>[2x]LNEQVNYTPQQRQYLESFIEKYVDKTKGSKQYTDETRFAHANNRNLSSFRSYWKEMVYP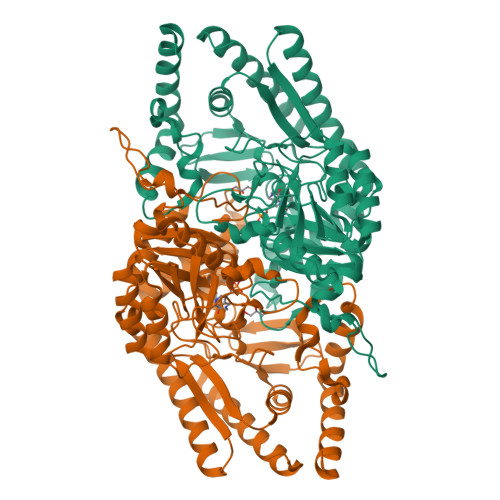IIAERSDGSRMWDIDGNEYIDITMGFGVNLFGHHPSFITQTVVDSTHSALPPLGPMSNVAGEVADRIRACTGVERVAFYNSGTEAVMVALRLARAATGRTKVVVFAGSYHGTFDGVLGVANTKGGAEPANPLAPGIPQSFMNDLIILHYNHPDSLDVIRNLGNELAAVLVEPVQSRRPDLQPESFLKELRAITQQSGTALIMDEIITGFRIGLGGAQEWFDIQADLVTYGKIIGGGQPLGIVAGKAEFMNTIDGGTWQYGDDSYPTDEAKRTFVAGTFNTHPLTMRMSLAVLRYLQAEGETLYERLNQKTTYLVDQLNSYFEQSQVPIRMVQFGSLFRFVSSVDNDLFFYHLNYKGVYVWEGRNCFLSTAHTSDDIAYIIQAVQETVKDLRRGGFIPEGPDS> EHCERLPYDASKWEFPRDRLKLGKPLGRGAFGQVIEADAFGIDKTATCRTVAVKMLKEGATHSEHRALMSELKILIHIGHHLNVVNLLGACTKPGGPLMVITEFCKFGNLSTYLRSKRNEFVPYKVAPEDLYKDFLTLEHLICYSFQV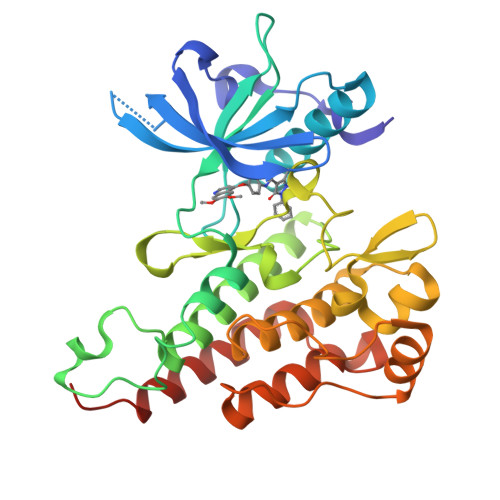AKGMEFLASRKCIHRDLAARNILLSEKNVVKICDFGLARDIYKDPDYVRKGDARLPLKWMAPETIFDRVYTIQSDVWSFGVLLWEIFSLGASPYPGVKIDEEFCRRLKEGTRMRAPDYTTPEMYQTMLDCWHGEPSQRPTFSELVEHLGNLLQANAQQDRHHHHHH1-(1-methyl-1,2,3,4-tetrahydroquinolin-6-yl)methanamine | C11 H16 N2 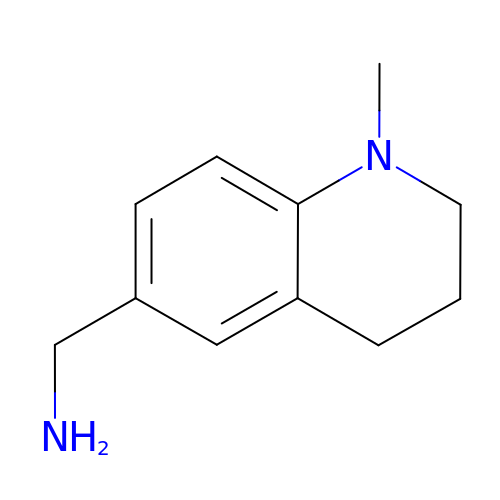| YWWOJPNCKNCDOR-UHFFFAOYSA-N>[4x]GSHMGVGSVAALLTVVFYIAAVMATNLYGATFPEWFGDLSKSLYTLFQVMTLDSWSMGIVRPVMNVHPNAWVFFIPFIMLTTFTVLNLFIGIIVDAMAITKEQEEEAKTGHHQEPI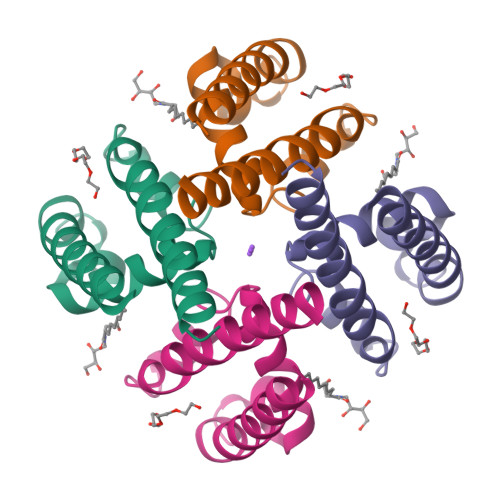SQTLLHLGDRLDRIEKQLAQNNELLQRQQPQKK>[7x]AYDRAITVFSP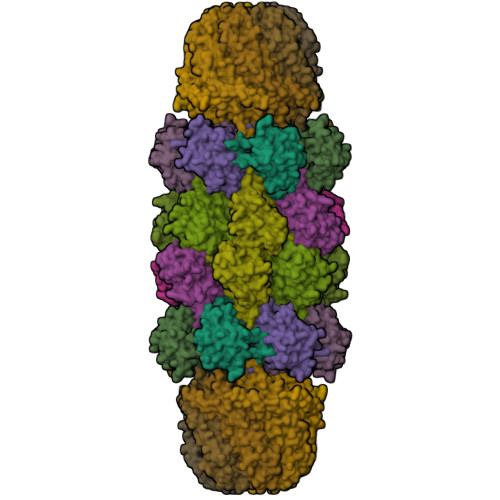DGRLFQVEYAREAVKKGSTALGMKFANGVLLISDKKVRSRLIEQNSIEKIQLIDDYVAAVTSGLVADARVLVDFARISAQQEKVTYGSLVNIENLVKRVADQMQQYTQYGGVRPYGVSLIFAGIDQIGPRLFDCDPAGTINEYKATAIGSGKDAVVSFLEREYKENLPEKEAVTLGIKALKSSLEEGEELKAPEIASITVGNKYRIYDQEEVKKFL;>TTTVGITLKDAVIMATERRVTMENFIMHKNGKKLFQIDTYTGMTIAGLVGDAQVLVRYMKAELELYRLQRRVNMPIEAVATLLSNMLNQVKYMPYMVQLLVGGIDTAPHVFSIDAAGGSVEDIYASTGSGSPFVYGVLESQYSEKMTVDEGVDLVIRAISAAKQRDSASGGMIDVAVITRKDGYVQLPTDQIESRIRKLGLIL[7x];>[7x]KRAALIQNLRDSYTETSSFAVIEEWAAGTLQEIEGIAKAAAEAHGVIRNSTYGRAQAEKSPEQLLGVLQRYQDLCHNVYCQAETIRTVIAIRIPEHKEEDNLGVAVQHAVLKIIDELEIKTLGSGEKSGSGGAPTPIGMYALREYLSARSTVEDKLLGSVDAESGKTKGGSQSPSLLLELRQIDADFMLKVELATTHLSTMVRAVINAYLLNWKKLIQPRTGTDHMFS> IVGGYTCGANTVPYQVSLNSGYHFCGGSLINSQWVVSAAHCYKSGIQVRLGEDNINVVEGNEQFISASKSIVHPSYNSNTLNNDIMLIKLKSAASLNSRVASISLPTSCASAGTQCLISGWGNTKSSGTSY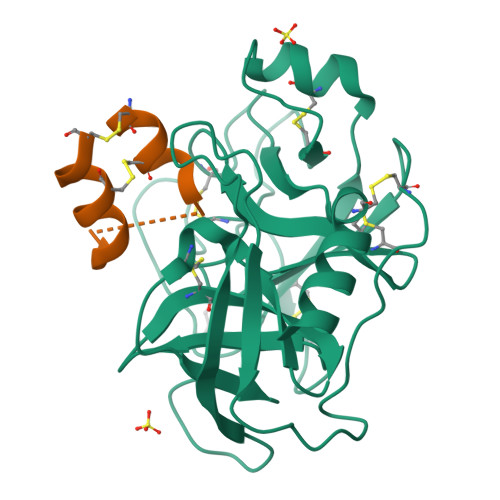PDVLKCLKAPILSDSSCKSAYPGQITSNMFCAGYLEGGKDSCQGDSGGPVVCSGKLQGIVSWGSGCAQKNKPGVYTKVCNYVSWIKQTIASN;> NTDPEQCKVMCYAQRHSSPELLRRCLDNCEKEHD>VQFRGGTTAQHATFTGAAREITVDTDKNTVVVHDGATAGGFPLARHDLVKTAFIKADKSAVAFTRTGNATASIKAGTIVEVNGKLVQFTADTAITMPALTAGTDYAIYVCDDGTVRADSNFSAPTGYTSTTARKVGGFHYAPGSNAAAQAGGNTTAQINEYSLWDIKFRPAALDPRGMTLVAGAFWADIYLLGVNHLTDGTSKYNVTIADGSASPKKSTKFGGDGSAAYSDGAWYNFAEVMTHHGKRLPNYNEFQALAFGTTEATSSGGTDVPTTGVNGTGATSAWNIFTSKWGVVQASGCLWTWGNEFGGVNGASEYTANTGGRGSVYAQPAAALFGGAWNGTSLSGSRAALWYSGPSFSFAFFGARGVCDHLIL[6x];>DWNNQSIIKAGERQHGIHIKQSDGAGVRTATGTTIKVSGRQAQGVLLENPAAELRFQNGSVTSSGQLFDEGVRRFLGTVTVKAGKLVADHATLANVSDTRDDDGIALYVAGEQAQASIADSTLQGAGGVRVERGANVTVQRSTIVDGGLHIGTLQPLQPEDLPPSRVVLGDTSVTAVPASGAPAAVSVFGANELTVDGGHITGGRAAGVAAMDGAIVHLQRATIRRGDAPAGGAVPGGAVPGGAVPGGFGPLLDGWYGVDVSDSTVDLAQSIVEAPQLGAAIRAGRGARVTVSGGSLSAPHGNVIETGGGARRFPPPASPLSITLQAGARAQGRALLYRVLPEPVKLTLAGGAQGQGDIVATELPPIPGASSGPLDVALASQARWTGATRAVDSLSIDNATWVMTDNSNVGALRLASDGSVDFQQPAEAGRFKVLMVDTLAGSGLFRMNVFADLGLSDKLVVMRDASGQHRLWVRNSGSEPASANTMLLVQTPRGSAATFTLANKDGKVDIGTYRYRLAANGNGQWSLVGAKAPP[2x]

Mtd is a pyramid-shaped trimeric protein that localizes to the ends of phage tail fibers and functions as the phage's receptor-binding protein. DGR-programmed variation of Mtd enables the phage to use alternative Bordetella receptors for infection. Variation in Mtd is focused on 12 adenine-encoded amino acids that are fixed in position and scattered across its C-terminal region. The 12 variable residues are organized into receptor-binding sites by the C-type lectin fold of Mtd.

We isolated, crystallized, and determined the structure of Mtd-P1 (120 kDa per trimer) bound to the 60 kDa ectodomain of B. bronchiseptica pertactin (Prn-E; residues 38–640). Structure determination to 3.16 Å resolution revealed that a single Mtd-P1 trimer, although possessing three independent receptor-binding sites, associated with just one Prn-E molecule. Two independent copies of the ∼180 kDa Mtd-P1·Prn-E complex occupied the asymmetric unit of the crystal. A total of ∼2300 Å2 was buried at the Mtd-P1·Prn-E interface. Two loops of pertactin emanating from its β-helix scaffold contacted Mtd. These loops nestled separately into two of the three receptor-binding sites of Mtd. The third receptor-binding site of Mtd was unoccupied and sterically occluded from binding another Prn-E molecule. One of the contacting pertactin loops, composed of residues 399–407, formed the majority of the interactions with a total of ∼870 Å2 being buried at this interface and was called the “major loop”. The other loop, composed of residues 190–199, made less extensive but nevertheless essential interactions (see below), with a total of ∼585 Å2 being buried at this interface, and was called the “minor loop”. Although the three separate and independent binding sites of Mtd-P1 interacted with different chemical environments, they were strikingly indistinguishable in conformation from one another and from unbound Mtd-P1.>[2x]MAEITETQESLPPFRMGEVGSLGLKVKNGRIYEEPRQALRFPESIKTFQLMMRDPAVAASVNIIKMFVRKVNWRFVPPKGKEQDPKMLERADFFNSLMDDMEHDWADFINSVMSFCTYGFCVNEKVYKKRQGKKGKYQSKFDDGLIGWAKLPIRNQSTLDKWYFDEDFRKVTGVRQNLRNVSHIAGAINLGERPLTRKLPRAKFMLFKYDDEYGNPEGRSPLLNAYVPWKYKVQIEEYEAVGVSRDLVGMPKIGLPPDYLDENAEPEKKAFVQYCKTVVNDMIANDRAGLIWPRYIDPDTKEDIFEFSLVSRQGAKAYDTGSIIDRYSKQIMMAFMSDVLAMGQSKYGSFSLADSKTSLLAMSVDILLKQIKNVINRDLVAQTYALNMWDDEEHVQITYDDIETPDLEAIGSYIQKTVAVGALEVDKELSNKLREHIGLPPADESQPVSEKLSPNSQSRSGDGYKTAGEGTAKTPSAKDPSTANKANK;>MCYTGDPANNPLDRVRILCTDTNNDEILIEQSVLEWFYLESGKDEKKAAIKALKYLLFQVAKMGDEKVGGVYLRNSSRFKSLKAVYDDLVKS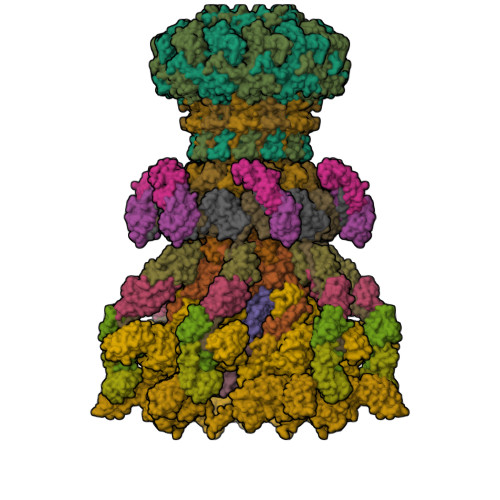SVSGLPYAGGINQCDIDMRRQNPCSVKKYTEYGDAARYEGRDYCNRVNGVFIIERDE[2x];> MRLLNRHSFVVKRKVSEDGYYNDDGDWVASQDIVEVNCKGNIQPYIKGSVKNGTQIALPEGIRLTDTRILYTTYKLRTSDDVEWNESDIVMIDGHEYEVFMTMDWSQQLAHTSHYEYIIIRRDKMNAVRNSRT;> MQLETAELEKGLVRTLVDVIGHRLARDKNNRPNVIRAYPSDNSNDKGLKPDQPFITVYCQDAATPYGWVLDKFVEDDVVCYRIAFQIPVLITVNGKGAHSIMLELKQRLEMSSVRDLILEETGATVLDTGAIPNDYTYLNTDFENSAPLVVTLVKNSVLKDERGSIIERVIVDGELVYEEGQEPPEYTIHLDVDSKGVK;>MAEVISISNATRVHSYRGVLIITDKLSVEAGSRASLSGYISDGGTSDVFTICRLLDAPMSGKPFISGNCSEIVKIPFDSSCLLGVKLYNCENKRINVNSIEAAFITLDTAFQSPMTVNKDTNRLEYIFSQNDYKVLVKGKVYDMIVNVVDESGNHSTVLKQKVRFN[2x];>MGTLTIDGKNKILATLTPTTIILHNVDPTADPTANKVTQPVAIYFSEPDNGLIASEDTVNITVPASATVSHYSLWDANDKCVATGALSKPQFFAEEGIYVISSVSVDLNK[6x];>[2x]MAMYQQYSPKDVVCSWNGIAIEGFAPDSFLRLQRTSPLVTPVVGAGGQVALTRNADKTGTIEIELMQTSLSNQMLSAIQAKQDNMELEEDISSNFVIYDPSGSVLATGINAWLQELPQIELGRDQNSKTWIFGCEKLDYTSTIPASSV;>MWNPIVNVDITLNTAGTTREGFGLPLFLASTDNFEERVRGYTSLTEVAEDFDENTAAYKAAKQLWSQTPKVTQLYIGRRAMQYTVSIPNAVTESTDYSITVAAGGGISQPYQYTAQAEDTAENVLQQFKTQIEADPTIKDKVSVNVTGSNGSATMIITKAGDNDFVKVTTTAQTVYIASTTADTASTALAAIEAYSTDWYFIAAEDRTQQFVLAMASEIQARKKIFFTANSDVTALQGTELASANDVPAQLAKNMYTRTVCLWHHAAAEDYPEMAYIAYGAPYDAGSIAWGNAQLTGVAASLQPSNQRPLTSIQKSALDVRHCNFIDLDGGVPVVRRGITSGGEWIDIVRGVDWLESDLKTSLRDLLINQKGGKITYDDTGITRIRQVIETSLQRAVNRNFLSSYTVNVPKASQVALADKKARILKDVTFAGILAGAILDVDLKGTVAYE[2x]2-{[4-(5-ethylpyrimidin-4-yl)piperazin-1-yl]methyl}-5-(trifluoromethyl)-1H-benzimidazole 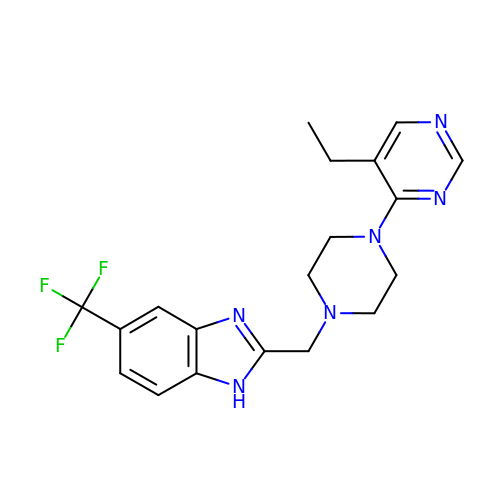| C19 H21 F3 N6 | FBLPQCAQRNSVHB-UHFFFAOYSA-N> GUGUGCCCGGCAUGGGUGCAGUCUAUAGGGUGAGAGUCCCGAACUGUGAAGGCAGAAGUAACAGUUAGCCUAACGCAAGGGUGUCCGUGGCGACAUGGAAUCUGAAGGAAGCGGACGGCAAACCUUCGGUCUGAGGAACACGAACUUCAUAUGAGGCUAGGUAUCAAUGGAUGAGUUUGCAUAACAAAACAAAGUCCUUUCUGCCAAAGUUGGUACAGAGUAAAUGAAGCAGAUUGAUGAAGGGAAAGACUGCAUUCUUACCCGGGGAGGUCUGGAAACAGAAGUCAGCAGAAGUCAUAGUACCCUGUUCGCAGGGGAAGGACGGAACAAGUAUGGCGUUCGCGCCUAAGCUUGAACCGCCGUAUACCGAACGGUACGUACGGUGGUGUGG

The self-splicing group II introns are bacterial and organellar ancestors of the nuclear spliceosome and retro-transposable elements of pharmacological and biotechnological importance. Besides catalyzing their self-splicing, group II introns also act as mobile retroelements, thus crucially contributing to genetic diversity throughout evolution. Integrating enzymatic, crystallographic, and simulation studies, we demonstrate how these introns recognize small molecules through their conserved active site. These RNA-binding small molecules selectively inhibit the two steps of splicing by adopting distinctive poses at different stages of catalysis, and by preventing crucial active site conformational changes that are essential for splicing progression.

To mimic a more physiological conformation of the active site immediately after 5’-exon hydrolysis, we thus co-crystallized OiD1-5 (the free intron) with the 5’-exon-like oligonucleotide 5’-AUUUAU-3’ in the presence of Mg2+ and K+, and we solved the X-ray structure of this complex in the absence of inhibitors, and in the presence of intronistat B or the di-brominated intronistat B derivative ARN25850 at different soaking time (1 h or 2.5 h). After 1 h soaking time, intronistat B binds the intron in its active site still coordinating M1 and M2 through its pyrogallol moiety. However, in this structure, the Fo-Fc omit map calculated before modeling the 5’-exon-like oligonucleotide substrate 5’-AUUUAU-3’ and the compound shows that the oligonucleotide is absent. B Crystal structure of OiD1-5 with Mg2+, K+, 5’-exon-like oligonucleotide 5’-AUUUAU-3’ (not resolved), and intronistat B (gray sticks) after 1 h soaking. The anomalous difference Fourier electron density map obtained collecting the data at λ = 0.92 Å shows two pronounced peaks (highest contour value = 7.3 σ and 8 σ, respectively) in the active site at the expected ortho positions on the pyrogallol moiety, unequivocally confirming the binding of inhibitor in the intron active site at this step of the catalytic cycle. These data demonstrate that intronistat B competes with the 5’-exon for binding the intron active site after the first splicing step.> MFQQLSARLQEAIGRLRGRGRITEEDLKATLREIRRALMDADVNLEVARDFVERVREEALGKQVLESLTPAEVILATVYEALKEALGGEARLPVLKDRNLWFLVGLQGSGKTTTAAKLALYYKGKGRRPLLVAADTQRPAAREQLRLLGEKVGVPVLEVMDGESPESIRRRVEEKARLEARDLILVDTAGRLQIDEPLMGELARLKEVLGPDEVLLVLDAMTGQEALSVARAFDEKVGVTGLVLTKLDGDARGGAALSARHVTGKPIYFAGVSEKPEGLEPFYPERLAGRILGMGDIESILEKVKGLEEYDKIQKKMEDVMEGKGKLTLRDVYAQIIALRKMGPLSKVLQHIPGLGIMLPTPSEDQLKIGEEKIRRWLAALNSMTYKELENPNIIDKSRMRRIAEGSGLEVEEVRELLEWYNNMNRLLKMVK;> AALALAAAAALALA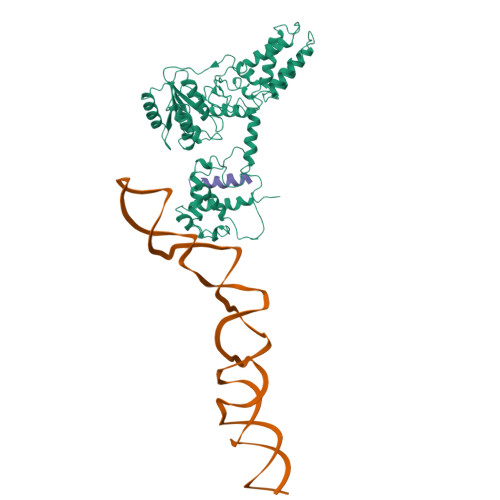AAG> GPGSEFMPKTISVRVTTMDAELEFAIQPNTTGKQLFDQVVKTIGLREVWFFGLQYQDTKAFSTWLKLNKKVTAQDVRKESPLLFKFRAKFYPEDVSEELIQDITQRLFFLQVKEGILNDDIYCPPETAVLLASYAVQSKYGDFNKEVHKSGYLAGDKLLPQRVLEQHKLNKDQWEERIQVWHEEHRGMLREDAVLEYLKIAQDLEMYGVNYFSIKNKKGSELWLGVDALGLNIYEQNDRLTPKIGFPWSEIRNISFNDKKFVIKPIDKKAPDFVFYAPRLRINKR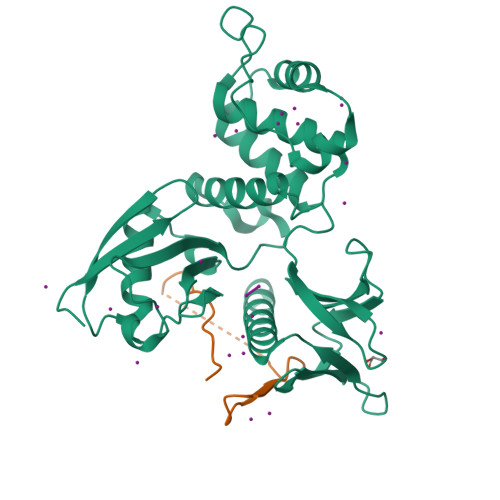ILALCMGNHELYMRRRKP;> GPGSEFRNKRATRGTYSPSAQEYCNPRLEMDNVLKPPPEERLI>[2x]SNASQEIVAGELERCFLAMPESVLPIVTMEERNDLCRRAGHLS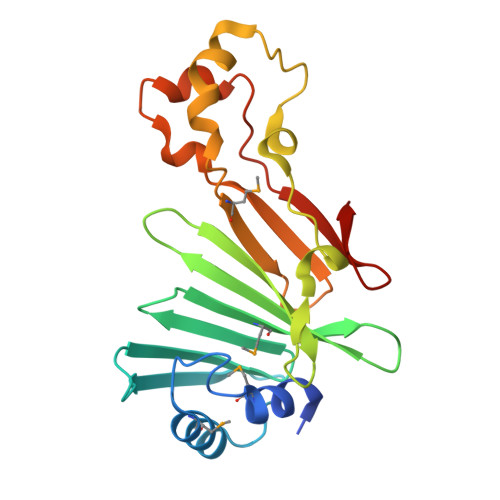GFTHTASLESSLGGTVTFLLNRNFIRIQTSTVGEVFMRILPFSDSSSVICVVTTVLHPVADSRIDFYTTEWKPLKTDRFWQQPRIEDFFLPHTDRQSYAYQAIYASLTPSYMQVSLSEESDTLSIRQTVTETLAEEEKPLAAIFLSPEPLVYRWQSGRFVRQVR4-amino-1-(3-deoxy-3-fluoro-beta-D-glucopyranosyl)pyrimidin-2(1H)-one | C10 H14 F N3 O5 | 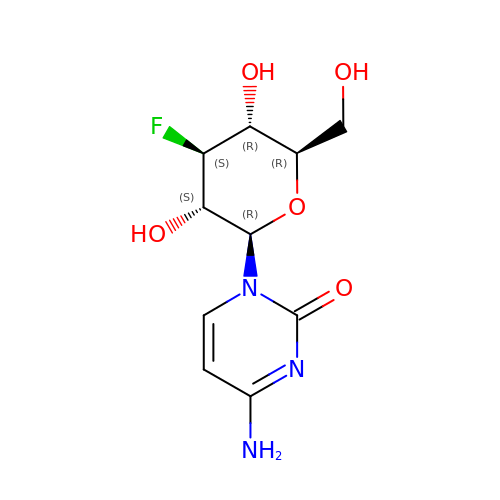AGFREDUIXIMAKC-PMPOVCSBSA-N>[3x]MNSQLTLRALERGDLRFIHNLNNNRNIMSYWFEEPYESFDELEELYNKHIHDNAERRFVVEDAQKNLIGLVELIEINYIHRSAEFQIIIAPEHQGKGFARTLINRALDY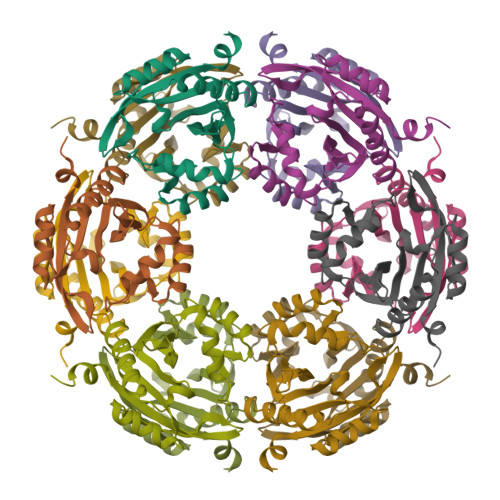SFTILNLHKIYLHVAVENPKAVHLYEECGFVEEGHLVEERLFKGRYQDVKRMYILQSKYLNRSE>IPNKRKPYKPCKNLVFYFHD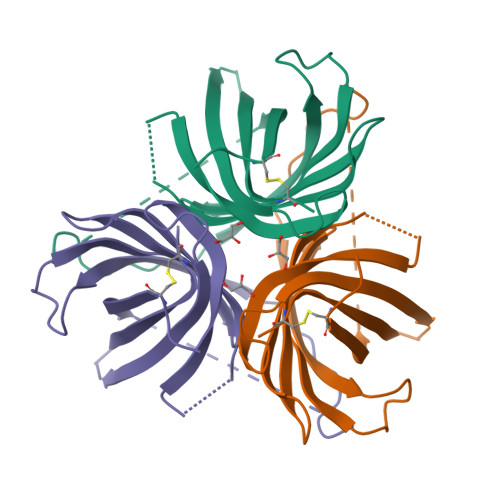ILYNGKNAANATSAIVAAPEGVSLTKLAPQSHFGNIIVFDDPITLSHSLSSKQVGRAQGFYIYDTKNTYTSWLSFTFVLNSTHHQGTITFAGADPIVAKTRDISVTGGTGDFFMHRGIATITTDAFEGEAYFRLGVYIKFFECW[2x]2-(benzyloxy)-4-(1H-pyrazol-4-yl)-N-(2,3,4,5-tetrahydro-1H-3-benzazepin-7-yl)benzamide 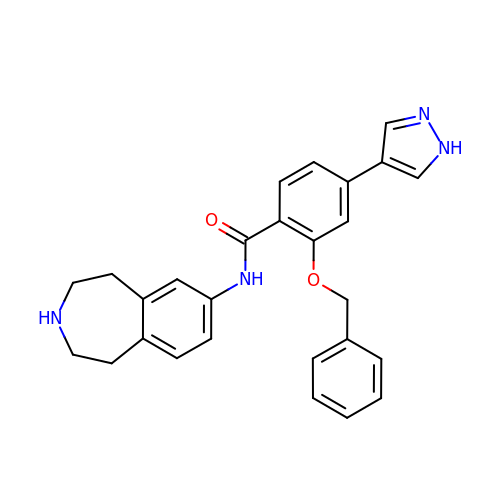| C27 H26 N4 O2 | CZXJXUACNMVIHE-UHFFFAOYSA-N> TSPQREATCTSEVSGCPKIYNPVCGTDGITYSNECVLCSENKKRQTPVLIQKSGPC;> VDDDDKIVGGYTCGANTVPYQVSLNSGYHFCGGSLINSQ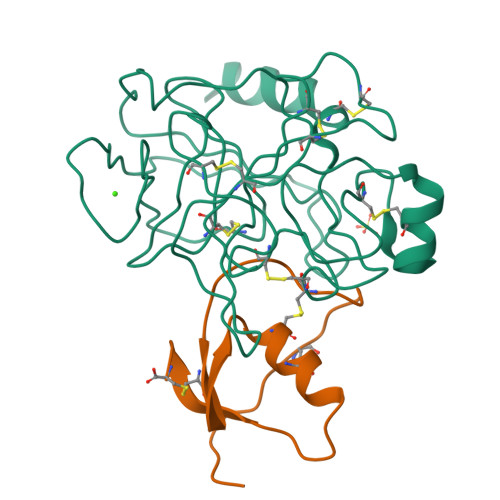WVVSAAHCYKSGIQVRLGEDNINVVEGNEQFISASKSIVHPSYNSNTLNNDIMLIKLKSAASLNSRVASISLPTSCASAGTQCLISGWGNTKSSGTSYPDVLKCLKAPILSDSSCKSAYPGQITSNMFCAGYLEGGKDSCQGDSGGPVVCSGKLQGIVSWGSGCAQKNKPGVYTKVCNYVSWIKQTIASN> EGELIPQVRIEDLKQMAAYLAHLAAQQAELNSLKAAHAAEHSTMQKLHCTQ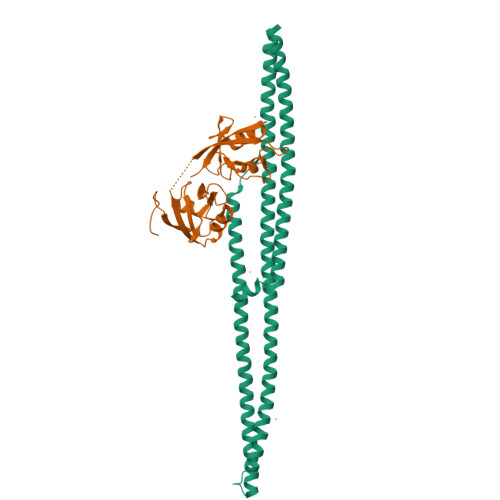VDKIVAQYDKEKSTHEKILEKAMKKKGGSNCLEIKKETEIKIQTLTTDHKSKVKEIVAQHTKEWSEMINTHSAEEQEIRDLHLSQQCELLRKLLINAHEQQTQQLKLSHDRESKEMRAHQAKISMENSKAISQDKSIKNKAERERRVRELNSSNTKKFLEERKRLAMKQSKEMDQLKKVQLEHLEFLEKQNEQAKEMQQMVKLEAEMDRRPATVV;> LSVDPATCPIVPGQEMIIEISKGRSGLGLSIVGGKDTPLNAIVIHEVYEEGAAARDGRLWAGDQILEVNGVDLRNSSHEEAITALRQTPQKVRLVVYRDEAHYRDEENLEIFPVDLQKKAGRGLGLSIVGKRNGSGVFISDIVKGGAADLDGRLIQGDQILSVNGEDMRNASQETVATILKCAQGLVQLEIGRLRAGSWTSARTTGGGSGGGGSGG>NLRGGAFVSNTQITMADKQKKFINEIQEGDLVRSYSITDETFQQNAVTSIVKHEADQLCQINFGKQHVVCTVNHRFYDPESK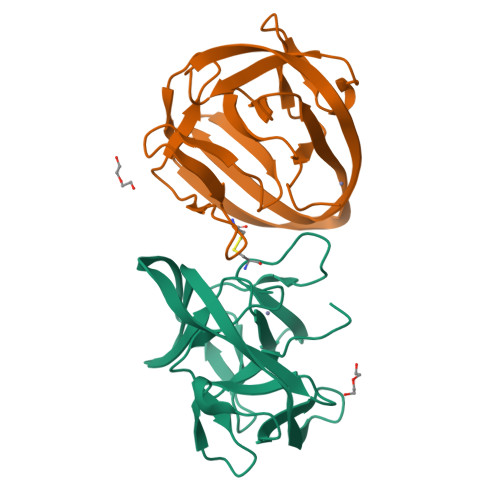LWKSVCPHPGSGISFLKKYDYLLSEEGEKLQITEIKTFTTKQPVFIYHIQVENNHNFFANGVLAHAMQVSI[2x];>NLRGGAFVSNTQITMADKQKKFINEIQEGDLVRSYSITDETFQQNAVTSIVKHEADQLCQINFGKQHVVCTVNHRFYDPESKLWKSVCPHPGSGISFLKKYDYLLSEEGEKLQITEIKTFTTKQPVFIYHIQVENNHNFFANGVLAHAMQ[2x]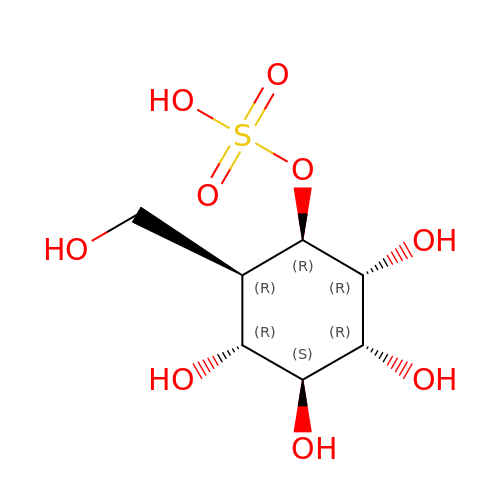[(1~{R},2~{R},3~{R},4~{S},5~{R})-2-(hydroxymethyl)-3,4,5,6-tetrakis(oxidanyl)cyclohexyl] hydrogen sulfate | C7 H14 O9 S | PDBNIRCVRHFXAD-XQCVOTFFSA-N> MSGELSNRFQGGKAFGLLKARQERRLAEINREFLCDQKYSDEENLPEKLTAFKEKYMEFDLNNEGEIDLMSLKRMMEKLGVPKTHLEMKKMISEVTGGVSDTISYRDFVNMMLGKRSAVLKLVMMFEGKANESSPKPVG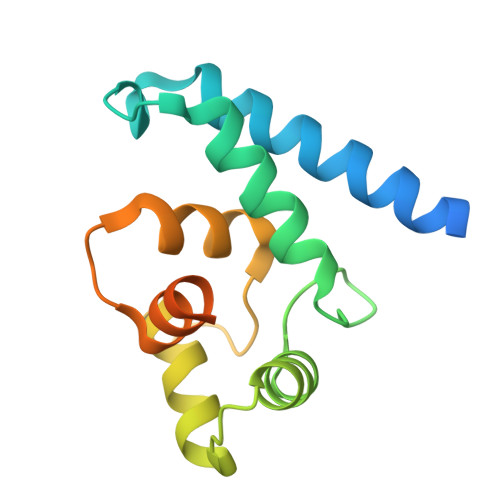PPPERDIASLP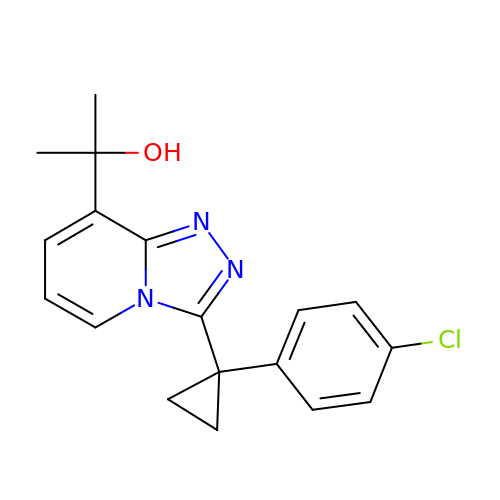2-{3-[1-(4-chlorophenyl)cyclopropyl][1,2,4]triazolo[4,3-a]pyridin-8-yl}propan-2-ol | C18 H18 Cl N3 O | PTIFVLOBVCIMKL-UHFFFAOYSA-N> ARKCSLTGKWTNDLGSNMTIGAVNSRGEFTGTYTTAVTATSNEIKESPLHGTENTINKRTQPTFGFTVNWKFSESTTVFTGQCFIDRNGKEVLKTMWLLRSSVNDIGDDWKATRVGINIFTRLRTQ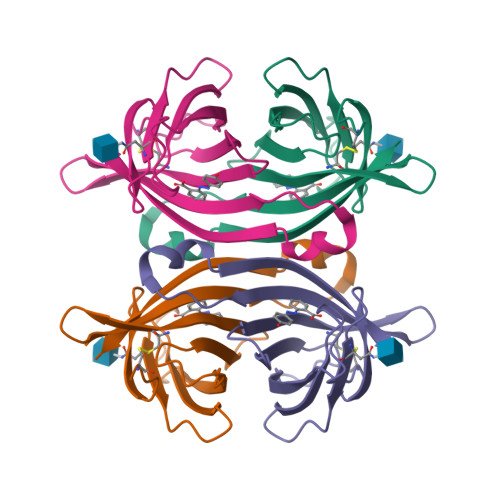KE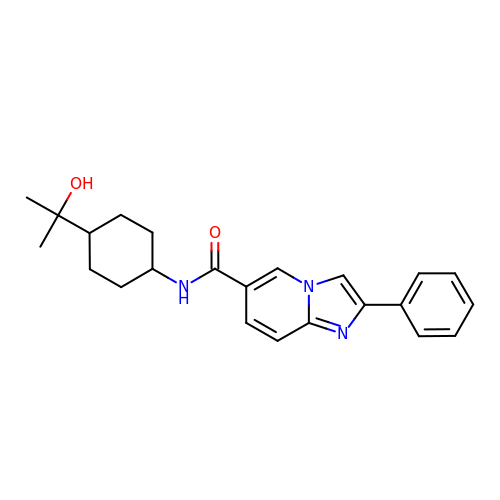N-[trans-4-(2-hydroxypropan-2-yl)cyclohexyl]-2-phenylimidazo[1,2-a]pyridine-6-carboxamide | C23 H27 N3 O2 | GOQZMCCBUBCPNK-WGSAOQKQSA-N>[2x]MNTTPVHALTDIDGGIAVDPAPRLAGPPVFGGPGNDAFDLAPVRSTGREMLRFDFPGVSIGAAHYEEGPTGATVIHIPAGARTAVDARGGAVGLSGGYDFNHAICLAGGAGYGLEAGAGVSGALLERLEHRTGFAELQLVSSAVIYDFSARSTAVYPDKALGRAALEFAVPGEFPQGRAGAGMSASAGKVDWDRTEITGQGA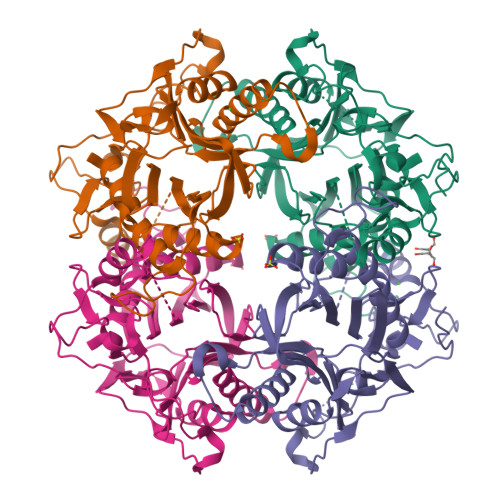AFRRLGDVRILAVVVPNPVGVIVDRAGTVVRGNYDAQTGVRRHPVFDYQEAFAEQVPPVTEAGNTTISAIVTNVRMSPVELNQFAKQVHSSMHRGIQPFHTDMDGDTLFAVTTDEIDLPTTPGSSRGRLSVNATALGAIASEVMWDAVLEAGK> GSLSWKRCAGCGGKIADRFLLYAMDSYWHSRCLKCS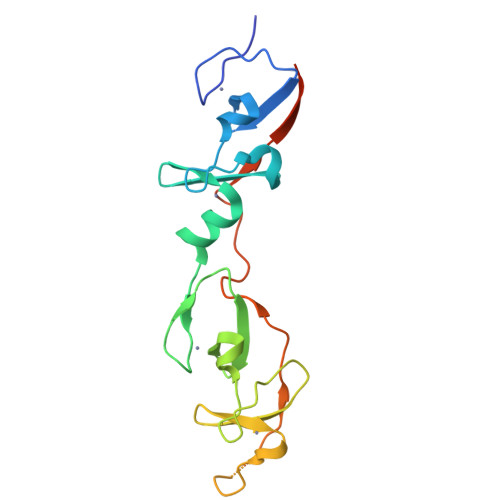SCQAQLGDIGTSSYTKSGMILCRNDYIRLFGNSGACSACGQSIPASELVMRAQGNVYHLKCFTCSTCRNRLVPGDRFHYINGSLFCEHDRPTALINGHLNSGGSGGSGGSGGDVMVVGEPTLMGGEFGDEDERLITRLENTQFDAANGIDDE> MEDKTLIKKRIDWFCKNKINAFSPTISPAPKSVERNEIESLYEGILWFVLNGVKEIVIEKKYMGSYCDIYLHRRLEDTYLVSRNGYKINHLDQEQCLRALQGLHDRFSWDGVELRIIQSELMPWSILGKGLINNEFSAYYISHEIHAEYLVQSSLYEKLQKIQQEPAYLSFVADAKV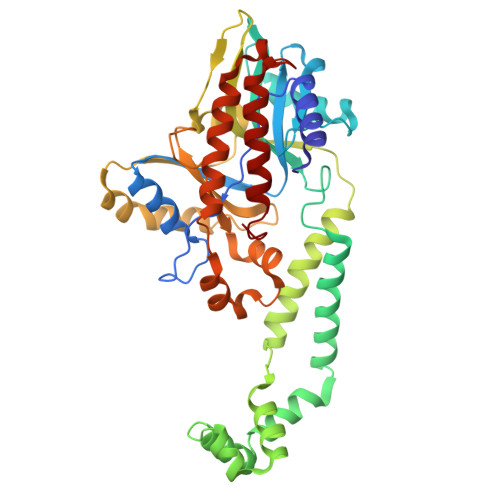LSAKELKDKYPMHIIRQYQSIRDFKFLDLPHYQQNIQLFKRQLDIFGKEAAPFFKPFNILKEVYTDGREHFVNDNLSFQQINDDDFLHYQFADREDFEAKYPQIRAWVDQVNQSDEEGVVIKPRTAFLPGMPPAFKVRNNDYLTLVYGVDFQDRLQEQIAKRNIKGKLRCSINDWAINAKLLAIPYSELGEENYELKNLVLDRILGEEIENQLDSRL>[2x]MECVKTRSVNIHVPVKETSKVVLECRGDSYFRHFSYVYWIIGKNKTVDQLPPNSGYRERIYLFKKPHRCENRPRADLILTNITDEMRNEKLTCVLIDPKDPLKESVILSKIWNCVYKI;>[2x]YFGKLESKLSVIRNLNDQVLFIDQGNRPLFEDMTDSDSRDNAPRTIFIISMYKDSQPRGMAVTISVASAAASTLSSENKIISFKEMNPPDNIKDTKSDIIFFQRSVPGHDNKMQFESSSYEGYFLASEKERDLFKLILKKEDELGDRSIMFTVQNED

IL18 is a pro-inflammatory cytokine belonging to the interleukin 1 superfamily and plays an important role in both innate and acquired immune responses by inducing interferon-γ (IFN-γ) production from T lymphocytes and macrophages while also enhancing the cytotoxicity of natural killer cells. Mammals and poxviruses encode homologous inhibitory proteins of IL18, named IL18BPs, which regulate IL18 activity and, in the case of the viral proteins, contribute to virulence. To understand the mechanism by which yatapoxvirus IL18BPs neutralize IL18, we solved the high-resolution crystal structure of the Yaba-Like Disease Virus (YLDV) IL18BP:IL18 complex. The structure of the complex shows that the YLDV-IL18BP forms a homo-dimer in a back-to-back fashion, with each protomer binding to a molecule of IL18, forming a hetero-tetramer complex with a stoichiometry of 2∶2.

We found that the use of an IL18 mutant [IL18 (8S), see Materials and Methods], containing substitutions of the four-cysteines with serines and substitutions of four surface residues opposite to the IL18BP binding interface with alanines, greatly improved crystal quality and reproducibility. The crystal structure of IL18 (8S) in complex with YLDV-IL18BP was determined to 2.7 Å. The two structures are essentially identical to each other with a root mean square deviation (r.m.s.d) of less than 0.4 Å, and the three mutated cysteines in YLDV-IL18BP are distant from the IL18 binding interface. YLDV-IL18BP contains five cysteine residues, forming two intra-molecular disulfide bonds (SS) (C21–C87, C43–C111) and one inter-molecular SS bond (C132–C132), in contrast to only two intra-molecular SS bonds in ECTV-IL18BP. The homo-dimer interface involves mainly βA, βB, βH and the C-terminal helix H3. It involves extensive hydrophobic interactions in the center (I29, H30, V31, P32 and V33 from βA, the aliphatic side chain of E122, V124 from βH and I129 from H3) flanked by hydrogen bonding and charge-charge interactions, burying approximately 1,700 Å2 and 1,465 Å2 solvent accessible surface area (ASA) for the wild-type complex and the triple-cysteine mutant complex, respectively. The inter-chain C132-C132 SS bond covalently links the two promoters. Indeed, a non-reducing SDS-PAGE showed that YLDV-IL18BP proteins expressed in E. coli or in mammalian cells formed disulfide-bonded dimers. In contrast, YLDV-IL18BP forms a disulfide-bonded dimer, which was demonstrated not only in the crystal structure but also in solution by non-reducing SDS-PAGE and gel filtration analysis. The dimer interface is quite large (about 1,700 Å2) and involves extensive hydrophobic interactions in addition to the intermolecular disulfide bond, indicating that the YLDV-IL18BP dimer is intrinsically stable in solution.> MFLGIFKDVIKLLNKKVVPVYFWFFLYCFLSTMDTNIFVSSCSFLKVEVFGKDENTTLVLLFYVFYSLFNFYLSRIK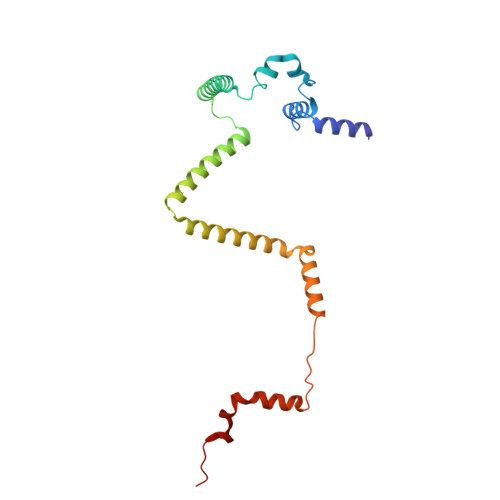NKNNYLVRKHLYTTELLIELILFKYKLIILKFSSIKYILNFNVRKFILFNLFLINNYKAYKINTFFLYIYIYLNNLNIIWYPIFKAYSIFGYYKSTRLNFIDTKNENIKRIKY L1 is a dizinc subclass B3 metallo-β-lactamase (MBL) that hydrolyzes most β-lactam antibiotics and is a key resistance determinant in the Gram-negative pathogen Stenotrophomonas maltophilia, an important cause of nosocomial infections in immunocompromised patients. We describe kinetic studies and crystal structures of L1 in complex with hydrolyzed β-lactams from the penam (mecillinam), cephem (cefoxitin/cefmetazole), and carbapenem (tebipenem, doripenem, and panipenem) classes. Despite differences in their structures, all the β-lactam-derived products hydrogen bond to Tyr33, Ser221, and Ser225 and are stabilized by interactions with a conserved hydrophobic pocket. All of the β-lactam derived products are bound in the dizinc active site, in a manner apparently stabilized by binding in a pocket containing four hydrophobic residues (Trp39, Phe160, Ile166, and Pro227; standard MBL numbering is used throughout) that are conserved amongst known L1 variants.

We characterized the binding to L1 of the hydrolyzed products of tebipenem and doripenem, which contain a 1β-methyl group, and panipenem, which has a β-hydrogen atom at C-1. All three products are apparently bound (at least predominantly) as their Δ1-imine tautomers, with C-2 sp3 hybridized and in the (S)-configuration. All of the respective C-2 substituents (R2-groups in Figs. 1 and S1) are directed toward the solvent and do not interact with the protein main chain, consistent with similar catalytic efficiencies across the carbapenem class. The tebipenem- and doripenem-derived products bind almost identically, with the C-6 carboxylate (formed on opening of the β-lactam ring) bridging the Zn ions, apparently replacing the catalytic water/hydroxide. The C-6 α-hydroxyethyl substituent is therefore rotated away from the Zn ions and is positioned to hydrogen bond with Tyr33. The pyrroline C-3 carboxylate interacts with Zn2 and with the side chain oxygen atoms of Ser221 and Ser225; the pyrroline N further interacts with Zn2. The carbapenem products were modeled as Δ1-imines, with (2S)-stereochemistry. Their binding mode is determined by the presence of a 1β-methyl substituent: the Zn-bridging hydroxide either interacts with the C-6 hydroxyethyl group (1β-hydrogen-containing carbapenems) or is displaced by the C-6 carboxylate (1β-methyl-containing carbapenems). As a consequence, 1β-methyl-carbapenems (doripenem, tebipenem, ertapenem) adopt binding mode one in interactions with L1. Boronates bind to NDM-1 similar to the products of 1β-methyl-carbapenems to L1 (binding mode 1), including interactions with Zn2 and displacement of the Zn-bridging hydroxide by the boronate oxygen, together with a concomitant increase in the Zn – Zn distance. The complexed products derived from tebipenem (after a 16 h soak), panipenem (8 h), doripenem (16 h), mecillinam (16 h), cefoxitin (23 h), and cefmetazole (22 h) could all be confidently modeled into Fo-Fc electron density.

> GPAEVPLPQLRAYTVDASWLQPMAPLQIADHTWQIGTEDLTALLVQTPDGAVLLDGGMPQMASHLLDNMKARGVTPRDLRLILLSHAHADHAGPVAELKRRTGAKVAANAESAVLLARGGSDDLHFGDGITYPPANADRIVMDGEVITVGGIVFTAHFMAGHTPGSTAWTWTDTRNGKPVRIAYADSLSAPGYQLQGNPRYPHLIEDYRRSFATVRALPCDVLLTPHPGASNWDYAAGARAGAKALTCKAYADAAEQKFDGQLAKETAGAR> DYGALYEGRNPGFYVEA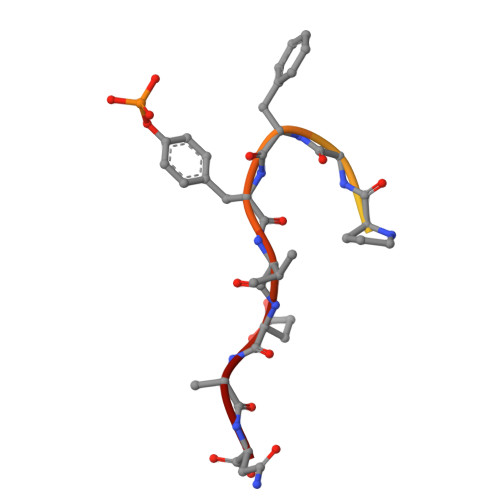N>[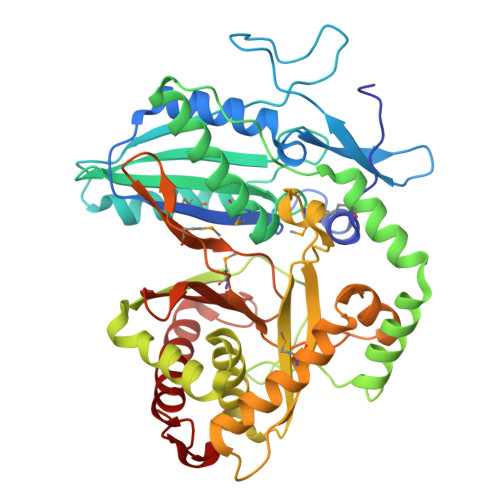2x]GMSENSSVRHGLTSAQHEVWLAQQLDPRGAHYRTGSCLEIDGPLDHAVLSRALRLTVAGTETLCSRFLTDEEGRPYRAYCPPAPEGSAAVEDPDGVPYTPVLLRHIDLSGHEDPEGEAQRWMDRDRATPLPLDRPGLSSHALFTLGGGRHLYYLGVHHIVIDGTSMALFYERLAEVYRALRDGRAVPAAAFGDTDRMVAGEEAYRASARYERDRAYWTGLFTDRPEPVSLTGRGGGRALAPTVRSLGLPPERTEVLGRAAEATGAHWARVVIAGVAAFLHRTTGARDVVVSVPVTGRYGANARITPGMVSNRLPLRLAVRPGESFARVVETVSEAMSGLLAHSRFRGEDLDRELGGAGVSGPTVNVMPYIRPVDFGGPVGLMRSISSGPTTDLNIVLTGTPESGLRVDFEGNPQVYGGQDLTVLQERFVRFLAELAADPAATVDEVALLT>MVNVAVIGAAGGIGQSLSLLLLRELPFGSTLSLYDVVGAPGVAADLSHIDRAGITVKHAAGKLPPVPRDPALTELAEGVDVFVIVAGVPRKPGMTRDDLFNVNAGIVMDLVLTCASVSPNACFCIVTNPVNSTTPIAAQTLRKIGVYNKNKLLGVSLLDGLRATRFINNARHPLVVPYVPVVGGHSDVTIVPLYSQIPGPLPDESTLKEIRKRVQVAGTEVVKAKAGRGSATLSMAEAGARFTMHVVKALMGLDTPMVYAYVDTDGEHECPFLAMPVVLGKNGIERRLPIGPITTVEKEMLEEAVGVVKKNIAKGETFARSKL[4x];> MDCSTGAAIGQQFAKDAFHMHGGVGVGPTGNSEHDVLMNEMMMVQTPTGPAGEWTHQFAAYQGQQQQQQQQHPQELAMRHQQNDAFMLRQQQEMEEAFCTFCTTHPHSHAHSHQPQGLVGPAMMGPQIMPPMMFGPGTGGFMMGAPPMMPYASMKFAGDAAMAAANNTNMTQGATATSTTSVQQELQQQSSDNGWVEKLRDAEWAQDYSDAQVFTLEGQSEQTMEEHAKNSEFYQFMDKIRSKELLIDEETGQLVQGPGPDPDAPEDAEYLKEWAAAEGLNMPPGFFEHMMQRPQGNNEQAEGRLFDGSNDALMDDGALDNAADVEEWVREYAEAQEQLQRVQNETNYPFEPNNPYMYHDKPMEEGIAMLQLANMAEAALAFEAVCQKEPENVEAWRRLGTTQAENEKDCLAIIALNHARMLDP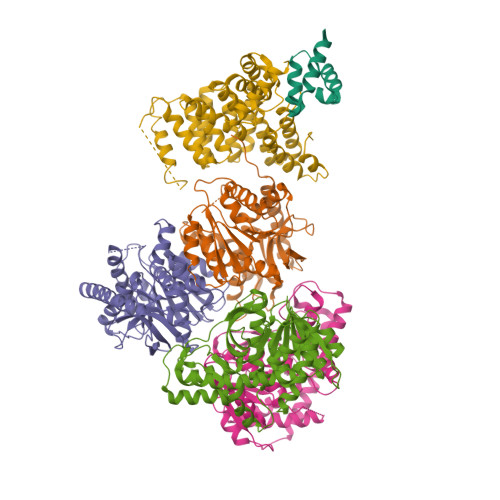KDIAVHAALAVSHTNEHNVGAALQSLRSWLLSQPQYEHLGLVDLREVAADEGLDEVPEENYFFAAPSEYRDCCTLLYAAVEMNPNDPQLHASLGVLHNLSHRFDEAAKNFRRAVELRPDDAHMWNKLGATLANGNRPQEALEAYNRALDINPGYVRVMYNMAVSYSNMAQYPLAAKHITRAIALQAGGTNPQGEGSRIATRGLWDLLRMTLNLMDRSDLVEASWQQDLTPFLREFGLEEMAV;> MNTATTVGVTGDGDARQRNSPEESEKRKRVSSAVQFLHDSRVKITPAANKIQFLKSKGLTTEEVCEAFEKAGQTIPLDEIKKIMNKPSFGQLGSGVVNNNLAPGHVGSDATYVLRQHPFMPHAGPLYTQQPPPFPQTPQGAKETDWRDVIIGVGAALISGFAAFKAFQIYSPYEIRRKDERTKKGSRMESQRRGKRHEGSVSPDRGAERPVTSLHTMAPPMPATPTPLPTATAANAAESTEREIQKLQSELKETQEALEKEKRSKAEISVSLGKLRGQINALSRTNDNLESRIKLLQEEVDKANSEANKRKELDASFTGAADGVPKSQSEDAIQPNGPPLLTPKILADTVGCNSAALNELPVLTAVEFVPEE>[2x]GSHMASSCAVQVKLELGHRAQVRKKPTVEGFTHDWMVFVRGPEHSNIQHFVEKVVFHLHESFPRPKRVCKDPPYKVEESGWAGFILPIEVYFKNKE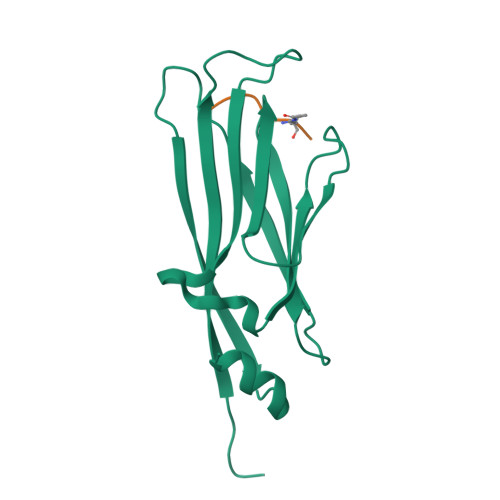EPRKVRFDYDLFLHLEGHPPVNHLRCEKLTFNNPTEDFRRKLLKA;>QTARXSSTGG[2x]6-[[(5-bromanylthiophen-2-yl)methyl-methyl-amino]methyl]-~{N}4-(4-methylphenyl)-1,3,5-triazine-2,4-diamine | C17 H19 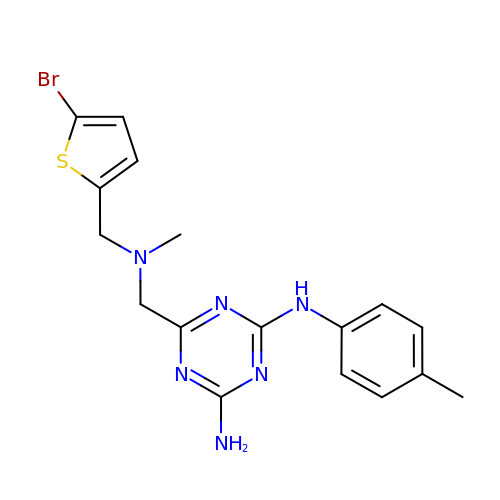Br N6 S | SDRWRCFYVVTRSA-UHFFFAOYSA-N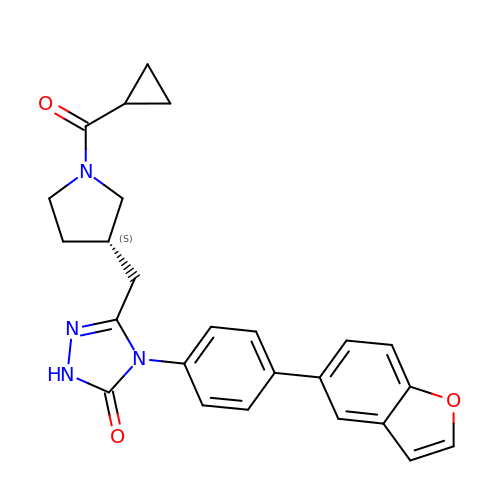4-[4-(1-benzofuran-5-yl)phenyl]-5-{[(3S)-1-(cyclopropylcarbonyl)pyrrolidin-3-yl]methyl}-2,4-dihydro-3H-1,2,4-triazol-3-one | C25 H24 N4 O3 | AQTPWCUIYUOEMG-INIZCTEOSA-N>SELLVYMNGEFVPESQAKVSVFDHGFLYGDGVFEGIRAYNGKVFKLYEHIDRLYDCARVIDLKIPLSKEEFAEAILETLRRNNLRDAYIRPIVTRGAGDLGLDPRKCPSPNVIIITKPWGKLYGDLYEKGLKAITVAIRRNAIDSLPPNIKSLNYLNNILAKIEANAKGGDEAIFLDHNGYISEGSGDNIFIVKNGTITTPPTLNNLKGITRQVVIELINELEIPFREANIGLFDLYSADEIFVTGTAAEIAPVTYIDGRTVGNGKPGKVTKMLMEKFRERTENEGVEIYR[3x]

Branched chain TAms (BCATs) catalyse reversible transamination of branched chain amino acids. The subunit of the archaeal BCATs has a PLP type IV fold typical of other BCATs, D-amino acid TAms and (R)-selective ωTAms and consists of two α/β domains, a small domain and a large domain connected by two inter-domain loops. A dimer formation is required for the BCAT catalytic activity, since residues from both subunits in the dimer contribute to the active site.

The GEO1900 holoform (internal aldimine form; GEO1900_holo) and the unproductive complex of holoenzyme with the keto substrate AKG-(GEO1900_AKG) have been determined to 1.9 and 2.2 Å resolution, respectively, in the trigonal space group P3221. The bound ligand AKG was found only in subunit A and was clearly defined in the electron density. A contact analysis reveals that α-carboxylic as well as α-keto groups of the ligand are tightly bound in the active site via hydrogen bonds with the highly conserved residues Tyr89, Ala249, Thr248, Arg91 as well as Ala250 and Gly188 (via a conserved water molecule D238). Although most of the residues around the γ-carboxylic group of the ligand are hydrophobic, this group is also connected to the protein via several hydrogen bonds with Arg91, Tyr29′ and Leu103′ (via the water molecule–D923). Comparative analysis of the holo form of GEO1900 and its complex with AKG reveals that the binding of the acceptor substrate does not result in any significant conformational changes in the active site, except for the rotation of the side chains of Leu101′ and Leu103′, accompanied by a small main chain displacement (distance between corresponding Cα-atoms is about 0.6 Å). In addition the AKG binding residues 120–124 of the inter-domain loop shift toward the active site. This positions the side chains of residues Trp120 and Leu123 so that they shield the ligand from the solvent. The structure of the complex GEO1900_AKG demonstrates that a major difference between the subunits can be assigned to a movement of the inter-domain loop which has a sufficiently different conformation in subunit A, where the ligand was bound, when compared to the other subunits. Thus, in the A subunit this loop adopts a conformation which shields the bound substrate from the solvent. As the residue displacements were only observed for the A subunit containing bound AKG, it is suggested that this could be the result of main-chain movement due to the substrate binding.> HMILKCILAFLLMVNEGWKMKILVRNLDRSVTEAEVLELFKAYGKVESCVVVTDKDTGKSKGFGFVEMPNPREAIKAIKGLNTLKVKGYGIRVKAAEE

Here, we identified an RRM-containing protein in Acinetobacter baumannii that we called AB-Elavl, starting from a protein similarity search with the human ELAV-like protein HuR. The single RRM domain is characterized by the presence of two consensus sequences: a highly conserved sequence (RNP1) of eight amino acids and a less conserved sequence of six (RNP2). The typical secondary structure consists of a β1α1β2β3α2β4 topology and the RNP1 and RNP2 are localized in the internal β1β3 strands. All these results suggest that A. baumannii express an RRM-containing RBP that shares RNA-binding properties and characteristics with the human HuR for the ability to bind RNA AU-rich region, although with lower affinity and specificity.

The crystals diffracted up to 1.6 Å resolution: they belong to space group I41 with one molecule in the asymmetric unit, a solvent content of about 50%, and a mosaicity of 0.3°. The X-ray structure showed the domain of an RRM domain: β1-α1-β2-β3-α2-β4 with an additional β5 segment present right before the C-terminus of the protein. The two conserved amino acid sequences, ILVNRL and KGFGFVE, are localized at the level of the two internal strands of the β-sheet: β2-β3. The solved structure shows the absence of the first 18 residues in the electron density with respect to the cloned sequence. It is not trivial to tell whether this is due to their high mobility or rather to their loss due to some protein degradation before/during crystallization. It appears quite clear that the fold of rAB-Elavl is very similar to that of the model used for structure solution and, in turn, similar to the typical RRM. The greatest discrepancy between the two structures is in the region involving residues from 50 to 58, just before RNP-1. In our case electron density is missing for those residues, confirming thus very high mobility. The average B-factor along the sequence is, in fact, about 35 Å2, confirming an overall rigidity of the structure, with the only exception being the above-mentioned region 50–58 where temperature factor values are extremely high. The structure of the bacterial RRM domain appears very similar to the eukaryotic one but for the presence of an additional short β strand and a more flexible central region.>GSPEEIRNLLADVETFVADTLKGENLSKKAKEKRESLIKKIKDVKSVYLQEFQDKGDAEDGDEYDDPFAGPADTISLASERYDKDDDGPSDGNQFPPIAAQDLPFVIKAGYLEKRRKDHSFLGFEWQKRWCALSKTVFYYYGSDKDKQQKGEFAIDGYDVRMNNTLRKDGKKDCCFEICAPDKRIYQFTAASPKDAEEWVQQ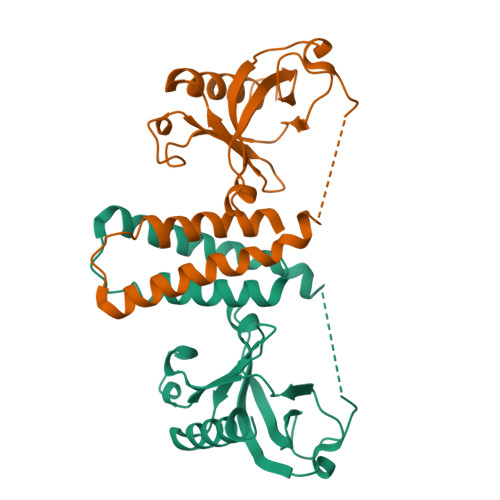LKFILQDLG[2x]> GAMDPRTITMHKDSTGHVGFIFKNGKITSIVKDSSAARNGLLTEHNICEIN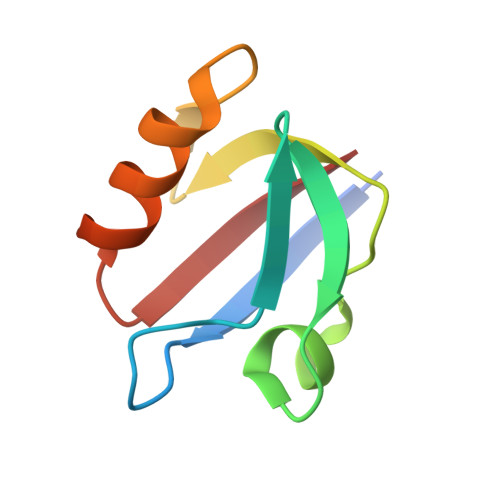GQNVIGLKDSQIADILSTSGTVVTITIM>MAFELPDLPYKLNALEPHISQETLEYHHGKHHRAYVNKLNKLIEGTPFEKEPLEEIIRKSDGGIFNNAAQHWNHTFYWHCMSPDGGGDPSGELASAIDKTFGSLEKFKALFTDSANNHFGSGWAWLVKDNNGKLEVLSTVNARNPMTEGKKPLMTCDVWEHAYYIDTRNDRPKYVNNFWQVVNWDFVMKNFKSENLY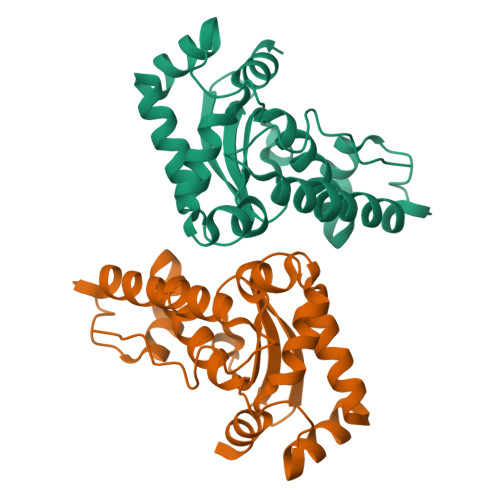FQGHHHHHHHHHH[2x]>GPSLDFALSLLRRNVRQVQTDQGHFTMLGVRDRLAVLPRHSQPGKTIWIEHKLVNVLDAVELVDEQGVSLELTLITLDTNEKFRDITKFIPENISTASDATLVINTEHMPSMFVPVGDVVQYGFLNLSGKPTHRTMMYNFPTKAGQCGGVVTSVGKIIGIHIGGNGRQGFCAGL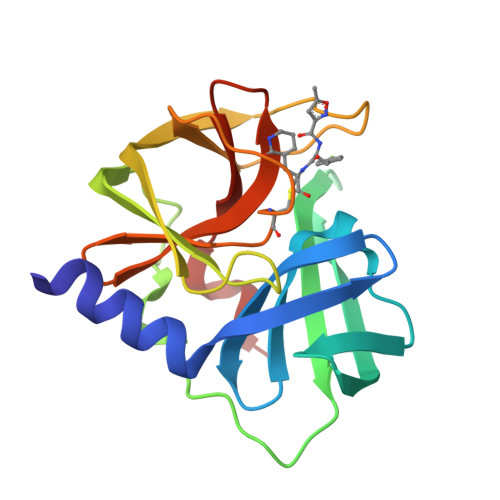KRSYFASEQ[5x]> MSLKHAVTGYWQNFNNGATVQKISDVPSAYDIIAVAFADATTTPGAVTFNLDSAGLGGYTVDQFKADVRAKQAAGKKVIISVGGEKGTVSVNSSASATNFANSVYSVMREYGFDGVDIDLENGLNPTYMTQALRALSAKAGPDMILTMAPQTIDMQSTQGGYFQTALNVKDILTVVNMQYYNSGTMLGCDGKVYAQGTVDFLTA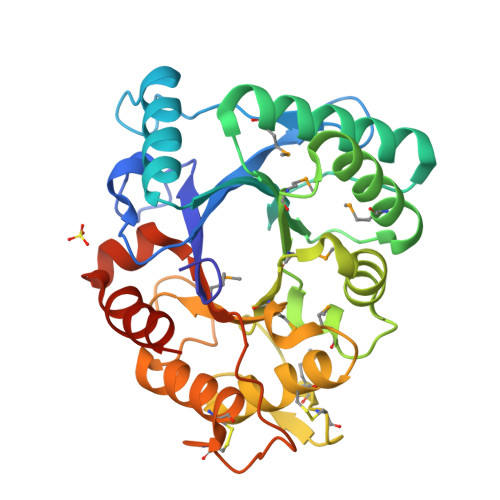LACIQLEGGLAPSQVGLGLPASTRAAGGGYVSPSVVNAALDCLTKATNCGSFKPSKTYPDLRGAMTWSTNWDATAGNAWSNSVGAHVHALEGHHHHHH The production of thiamine pyrophosphate (TPP), catalyzed by TPK, is critical for both catabolic and anabolic cellular processes. In yeast, this thiamine phosphate is then hydrolyzed into thiamine before pyrophosphorylation by the TPK that catalyzes the transfer of a pyrophosphate (PPi) from ATP to thiamine, resulting in AMP and TPP. CA1462 is a homodimer, with each monomer constituted of two domains.

The strong electronic density is consistent with thiamine molecules present at the thiamine binding site. The thiamine ammonium group N4 of the amidopyrimidine ring is engaged in a salt bridge with the Q138A main-chain carbonyl oxygen. The opposite side of this ring is stabilized by another salt bridge involving N1 and the oxygen from the S299B side chain. As observed in the mouse TPK/TPP complex, an Mg2+ ion is maintained by electrostatic interactions with the side chain of the four strictly conserved aspartate residues (D78, D113A, D115, D142). Interestingly, the C. albicans TPK/thiamine complex reveals a second Mg2+ partially stabilized by the hydroxyl group O1 of thiamine and a salt bridge with D113 and D142 side chains and with two main chain carboxy oxygens (Y140, N141). The nitrogen atom from the K145 side chain participates in the last coordination (Mg2+ number 2). As proposed by Timm et al., this lysine could be involved in the activation of the thiamine hydroxyl by the stabilization of a water molecule or, as in this C. albicans structure, of a magnesium ion. In the C. albicans thiamine complex, 2 water molecules take the place of oxygen atoms from the proximal thiamine phosphate. The equivalent glutamine (Q206A) adopts the same conformation in the C. albicans TPK/thiamine complex and an opened conformation in the C. albicans TPK/TPNP complex. The structure containing thiamine only exhibits the closed conformation, while both are present in the TPK/TPNP complex.

>[2x]MAHHHHHHGHHHQLSEDSELIEQVIEQPDSLIISPPSDSSSSSYNHIQPFVYLESTATTQTNHNVLLILNQKITIDLISLWKKCEIIVCADGGANSLYEYFNDNNHHHHHENLQRSDYIPDYIVGDFDSISPDVKTYYESHGSKIIRQSSQYYNDFTKSIHCIQLHYQLNHTKENWFESIDEVDGLAKLWNGLNNSSDVVVDIDITIYVLNAIGGRFDQTVQSINQLYIMNEDYPKVTVFFITTNDIIFLLKKGVNYISYKNRLMFHKDNGSSPTPTCGLLPLSNKTPIILNSYGLKYDMRNWKTEMLGQVSSSNRISGETGFIVECSDDIVMNIEIDV>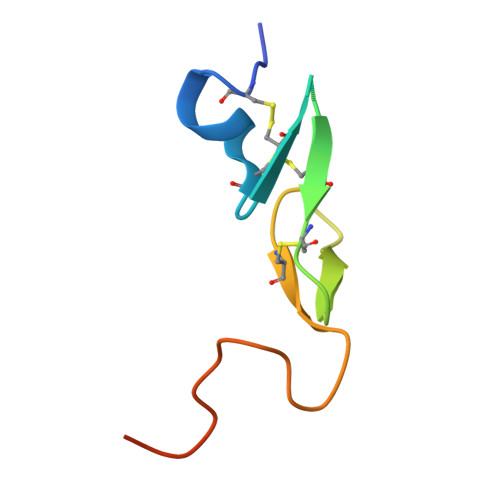 MDVTCNIKNGRCEQFCKNSADNKVVCSCTEGYRLAENQKSCEPAVPFPCGRVSVSQTSKLTR>MEHVAFGS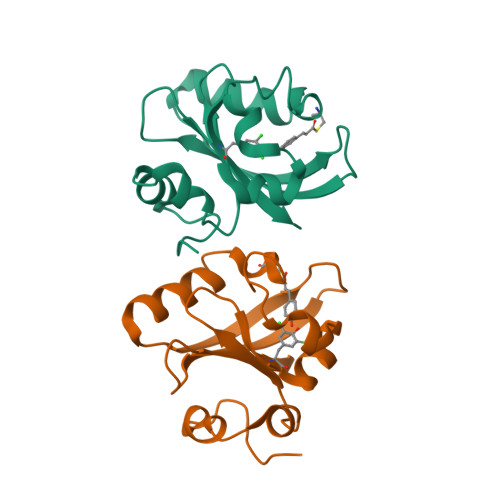EDIENTLAKMDDGQLDGLAFGAIQLDGDGNILQXNAAEGDITGRDPKQVIGKNFFKDVAPCTDSPEFYGKFKEGVASGNLNTMFEYTFDYQMTPTKVKVHMKKALSGDSYWVFVKRV[2x]> GAMGGSEF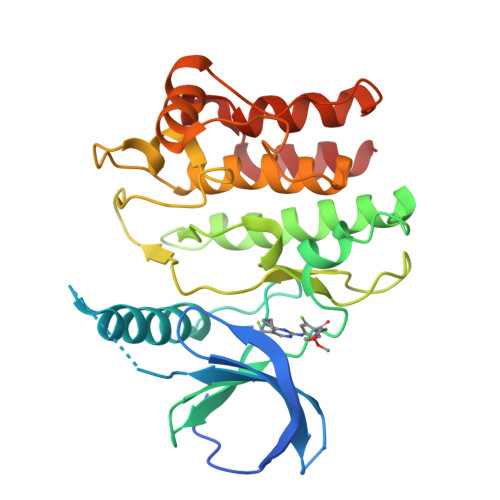PKSRLPTLADNEIEYEKQIGKGGFGLVHKGRLVKDKSVVAIKSLILGDSEGETEMIEKFQEFQREVFIMSNLNHPNIVKLYGLMHNPPRMVMELVPCGDLYHRLLDKAHPIKWSVKLRLMLDIALGIEYMQNQNPPIVHRDLRSPNILLQSLDENAPVCAKVADFGLSQQSVHSVSGLLGNFQWMAPETIGAEEESYTEKADTYSFAMILYTILTGEGPFDEYSYGKIKFINMIREEGLRPTIPEDCPPRLRNVIELCWSGDPKKRPHFSYIVKELSEL> GPGGTAINEPLTAAPIPVLRAVDTTSPNIVADTSTDREQRTFATQGGSVKPFTITKPSPYIPGLMLTNQEILYQAPDGKYYDFGTYNTLIMPSSSTSARVLPNSHPMQPLDSGGKMIACCTNQ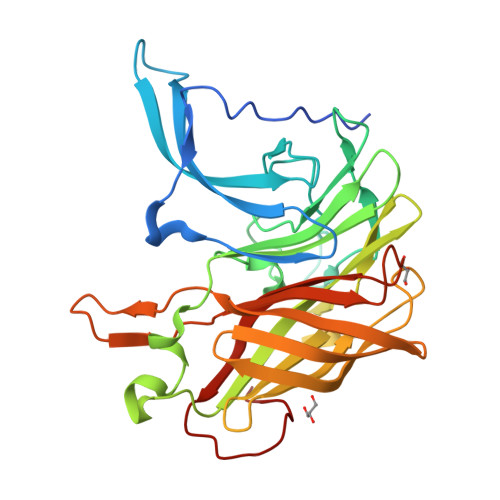TSTGMNALRLKSMQFGAWMSPSKTVSLFAGGTPAPTDTLQGVDTAGRPTGKATYEVIGLRVKNDRAVTSSYETRYSPYNTGQVVTGSFLTVNFNTGKLGGTIVGNSEFGDSIEMRDVNVNGNQFSGTASSGGHTGQVSGGLFAKEERFYSGTLEHPSGGEIGGTVNFGSNSPLNASFGGTRREYNAADTSTDTSHLVSPX>[4x]SQSRIFYLRNFNNWMKSVLIGEFLEKVRQKKKRDITVLDLGCGKGGDLLKWKKGRINKLVCTDIADVSVKQCQQRYEDMKNRRDSEYIFSAEFITADSSKELLIDKFRDPQMCFDICSCQFVCHYSFESYEQADMMLRNACERLSPGGYFIGTTPNSFELIRRLEASETESFGNEIYTVKFQKKGDYPLFGCKYDFNLEGVVDVPEFLVYFPLLNEMAKKYNMKLVYKKTFLEFYEEKIKNNENKMLLKRMQALEPYPANESSKLVSEKVDDYEHAAKYMKNSQVRLPLGTLSKSEWEATSIYLVFAFEKQQ

The cap intermediate is methylated by the RNA guanine N-7 methyltransferase, utilising the methyl donor, AdoMet, to create the mature cap, m7GpppN, and byproduct, AdoHcy (S-adenosyl homocysteine). In mammals, RNA guanylyltransferase and 5′-triphosphatase (RNGTT/CE) caps the nascent transcript and RNA guanine-7 methyltransferase (RNMT) methylates the cap. Human RNMT is a 476 amino acid nuclear protein consisting of a catalytic domain (residues 121–476), with homology to other eukaryotic cap methyltransferases and an N-terminal regulatory domain (residues 1–120), that mediates recruitment to transcription initiation sites. RNMT also has an activating subunit, RAM (RNMT-activating miniprotein).

Whilst high quality diffraction data (2.3 Å) was obtained, the lack of density in the lobe region indicated that the lobe was absent in the protein crystals. Moreover, only low quality crystals of the RNMT 165–476 monomer could be obtained using sparse matrix screens without proteolysis. Thus, binding of RAM permits stabilisation of a lobe structure, RNMT 416–456. RAM binding, however, stabilises the RNMT lobe (residues 416–456), a domain missing from structures of RNMT monomers. Despite the absence of the lobe in this mutant and in thermolysin-cleaved RNMT, the crystal structures are not altered significantly compared to RNMT–RAM (RMSD 0.5 Å). RAM binds distal to the RNMT active site and does not alter its crystal structure substantially when compared to the RNMT monomer or the E. cuniculi methyltransferase Ecm1 (15).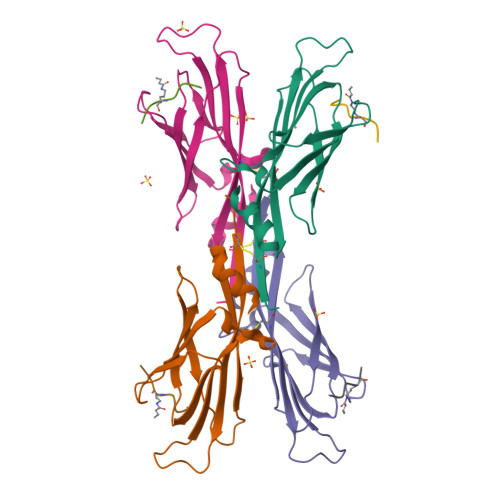>[8x]SHMASSCAVQVKLELGHRAQVRKKPTVEGFTHDWMVFVRGPEHSNIQHFVEKVVFHLHESFPRPKRVCKDPPYKVEESGYAGFILPIEVYFKNKEEPRKVRFDYDLFLHLEGHPPVNHLRCEKLTFNNPTEDFRRKLLKA;>KAPRXQL[8x]>GSHMSSRHQFAPGATVLYKGDKMVLNLDRSRVPTECIEKIEAILKELEKPAP[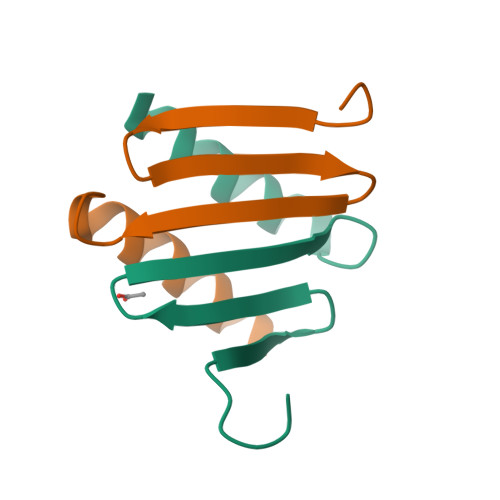3x]4-DIPHOSPHOCYTIDYL-2-C-METHYL-D-ERYTHRITOL | C14 H25 N3 O14 P2 | 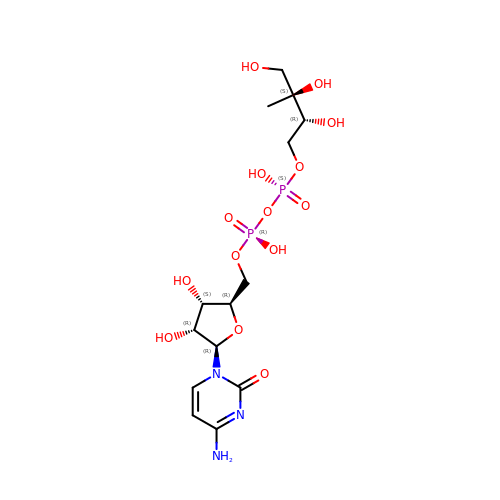YFAUKWZNPVBCFF-XHIBXCGHSA-N4,4'-(pyrimidine-2,4-diyldiimino)dibenzoic acid | C18 H14 N4 O4 | 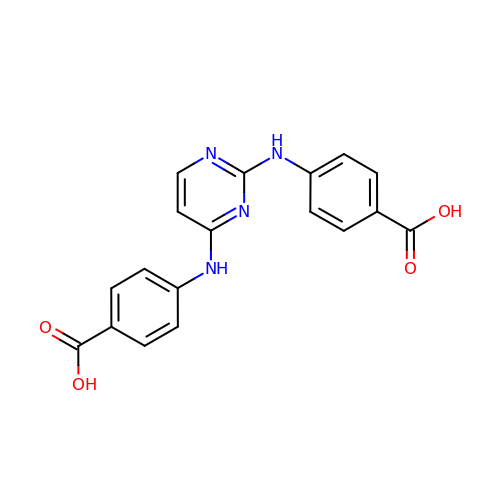PZRUXYWYONKHDD-UHFFFAOYSA-N> GP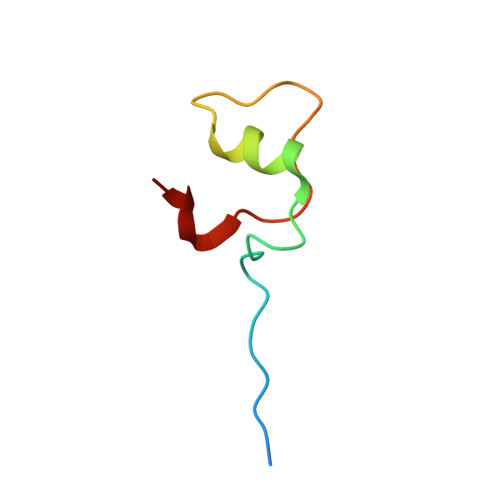SGSIIATDNVLFTPRDKLTVEELEQFQSKKFTLGKIPLKPPPLELLN>[4x]MCPQKLTISWFAIVLLVSPLMAMWELEKDVYVVEVDWTPDAPGETVNLTCDTPEEDDITWTSDQRHGVIGSGKTLTITVKEFLDAGQYTCHKGGETLSHSHLLLHKKENGIWSTEILKNFKNKTFLKCEAPNYSGRFTCSWLVQRNMDLKFNIKSSSSSPDSRAVTCGMASLSAEKVTLDQRDYEKYSV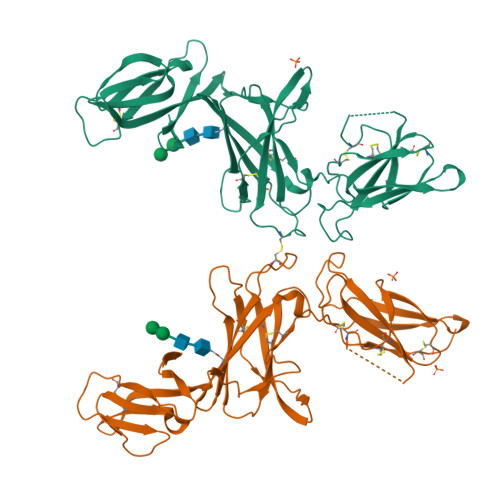SCQEDVTCPTAEETLPIELALEARQQNKYENYSTSFFIRDIIKPDPPKNLQMKPLKNSQVEVSWEYPDSWSTPHSYFSLKFFVRIQRKKEKMKETEEGCNQKGAFLVEKTSTEVQCKGGNVCVQAQDRYYNSSCSKWACVPCRVRS> MALRSAQGDGPTSGHWDGGAEKADFNAKRKKKVAEIHQALNSDPTDVAALRRMAISEGGLLTDEIRRKVWPKLLNVNANDPPPISGKNLRQMSKDYQQVLLDVRRSLRRFPPGMPEEQREGLQEELIDIILLILERNPQLHYYQGYHDIVVTFLLVVGERLATSLVEKLSTHHLRDFMDPTMDNTKHILNYLMPIIDQVNPELHDFMQSAEVGTI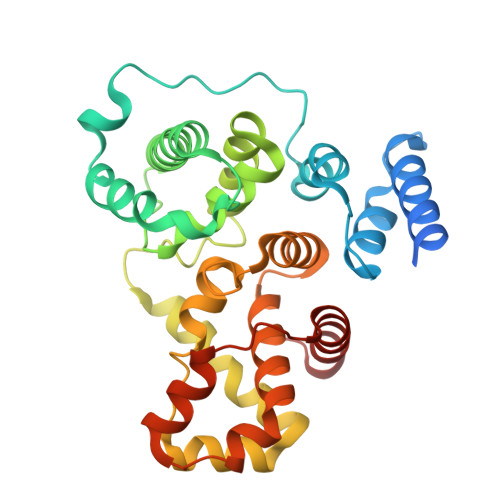FALSWLITWFGHVLSDFRHVVRLYDFFLACHPLMPIYFAAVIVLYREQEVLDCDCDMASVHHLLSQIPQDLPYETLISRAGDLFVQFPPS>[2x]GSMAEGRGSRERPDVETQKTELGALMGTTLQRGAQWYLIDSRWFKQWKKYVGFDSWDMYNVGEHNLFPGPIDNSGLFSDPESQTLKEHLIDELDYVLVPAEAWNKL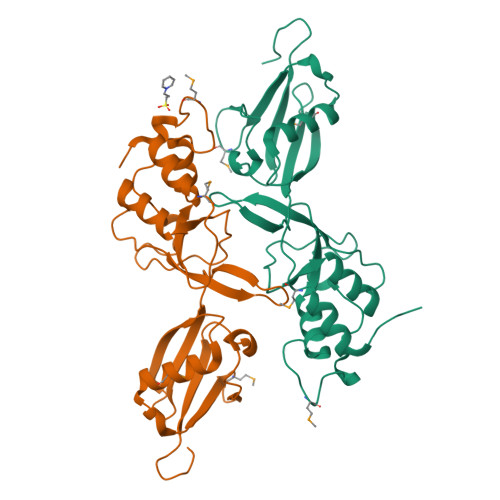LNWYGCVEGQQPIVRKVVEHGLFVKHCKVEVYLLELKLCENSDPTNVLSCHFSKADTIATIEKEMRKLFNIPAERETRLWNKYMSNTYEQLSKLDNTIQDAGLYQGQVLVIEPQNEDGTWPRQSL> MACAAARSPAEQDRFICIYPAYLNNKKTIAEGRRIPISKAVENPTATEIQDVCSAVGLNVFLEKNKMYSREWNRDVQYRGRVRVQLKQEDGSLCLVQFPSRKSVMLYAAEMIPKLKTRTQK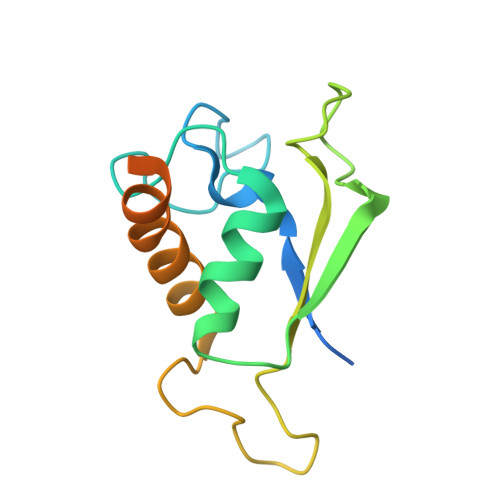TGGGDQSLQQGEGSKKGKGKKKK>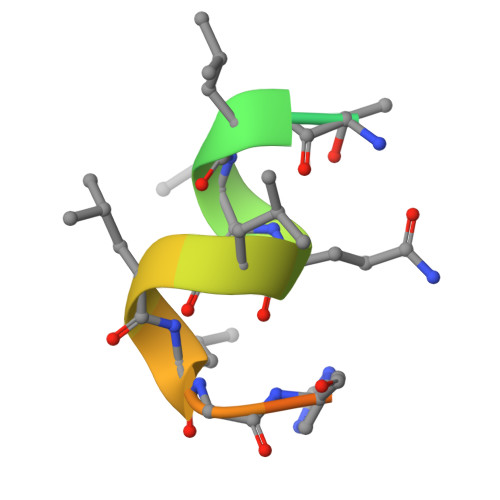 NSHQKVTLLQLLLGHKNEEN>[2x]GLNPPSAFSGAALACLEKMQASGVEEKCIHIFLIQHALVRKGETGYIPEKSISPV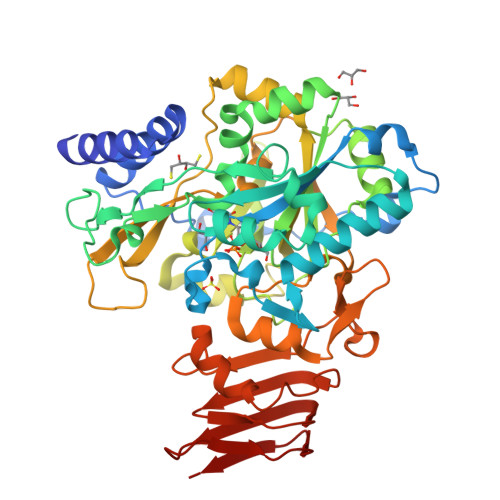ESLPFLQGIETKGENTALLRQAVVLKLNGGLGTGMGLNGPKSLLQVKNGQTFLDFTALQLEHFRQVRNCNVPFMLMNSFSTSGETKNFLRKYPTLYEVFDSDIELMQNRVPKIRQDNFFPVTYEADPTCEWVPPGHGDVYTVLYSSGKLDYLLGKGYRYMFISNGDNLGATLDVRLLDYMHEKQLGFLMEVCRRTESDKKGGHLAYKDVIDETTGQTRRRFVLRESAQCPKEDEDSFQNIAKHCFFNTNNIWINLMELKKMMDEQLGVLRLPVMRNPKTVNPQDSQSTKVYQLEVAMGAAISLFDRSEAVVVPRERFAPVKTCSDLLALRSDAYQVTEDQRLVLCEERNGKPPAIDLDGEHYKMIDGFEKLVKGGVPSLRQCTSLTVRGLVEFGADVSVRGNVVIKNLKEEPLIIGSGRVLDNEVVVVE N-{1-[(1-carbamoylcyclopropyl)methyl]piperidin-4-yl}-N-cyclopropyl-4-[(1S)-2,2,2-trifluoro-1-hydroxy-1-methylethyl]benzamide 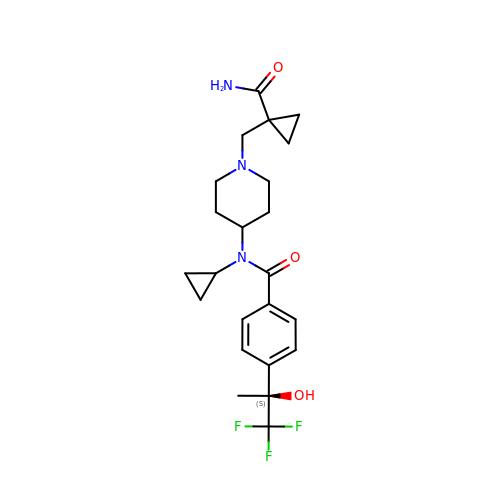| C23 H30 F3 N3 O3 | FAVXIEFZKPJZRT-NRFANRHFSA-N>[2x]GTNRRQNRKCGACAACLRRMDCGRCDFCCDKPKFGG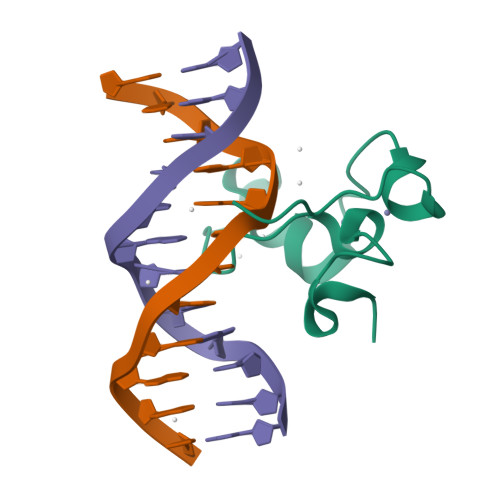SNQKRQKCRWRQCLQFAMKRLLPS>HHHHHHMIVLFVDFDYFYAQVEEVLNPSLKGKPVVVCVFSGRFEDSGAVATANYEARKFGVKAGIPIVEAKKILPNAVYLPMRKEVYQQVSSRIMNLLREYSEKIEIASIDEAYLDISDKVRDYREAYNLGLEIKNKILEKEKITVTVGISKNKVFAKIAADMAKPNGIKVIDDEEVKRLIRELDIADVPGIGNITAEKLKKLGINKLVDTLSIEFDKLKGMIGEAKAKYLISLARDEYNEPIRTRVRKSIGRIV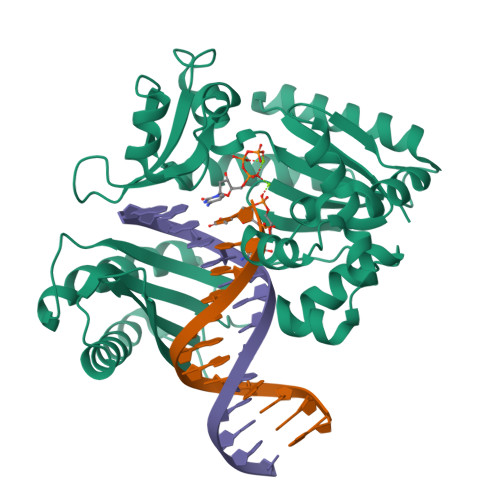TMKRNSRNLEEIKPYLFRAIEESYYKLDKRIPKAIHVVAVTEDLDIVSRGRTFPHGISKETAYSESVKLLQKILEEDERKIRRIGVRFSKFIEAIGLDKFFDT[2x]> MQMAKVCGTVVGTQKLPSMTGVKLLLLQFIDANGELLPKYEVAADPVGAGLGEWVLVNRGSAARQTEYHQNRPLDAMVVAIIDTVTVNNRRLYGEG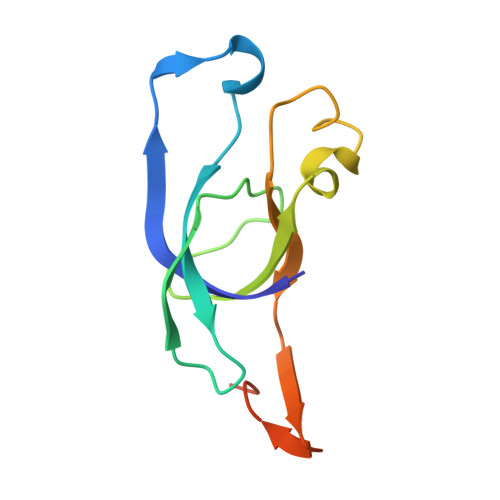SWSHPQFEK> MESAGPGTGPQPPRTSGDFTPDTGVIAEMTGRPMRFDSDRYRPTDTYAEVACDKVCRAYEGLGADGGDRESLLAFLRDLTDPWGELPVGTPPEDACWVSIDGMPLETSVAWAGRKAGVRLSLESPRGPAKRRMEDGMALTRRLAGRPGVSVDPCLRVEDLFTDDDPQGYFTIAHAVAWTPGGHPRYKIFLNPAVRGREQAAARTEEAMIRLGLEQPWR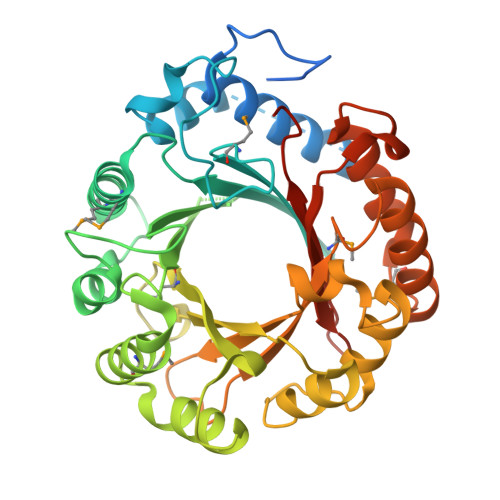ALTEHLGGAYGPEHEPAALAMDLVPGDDFRVQVYLAHSGVSAEAIDAKSAVAADHVPGSFARALRGINGADDTPEWKRKPPVTAFSFGPGRAVPGATLYVPMIPVHGSDAAARDRVAAFLRSEGMDAVGYEAVLDAISDRSLPESHTQNFISYRGGDSPRFSVYLAPGVYREALEHHHHHH(2E)-2-[(E)-({3-hydroxy-2-methyl-5-[(phosphonooxy)methyl]pyridin-4-yl}methylidene)amino]pent-2-enoic acid | C13 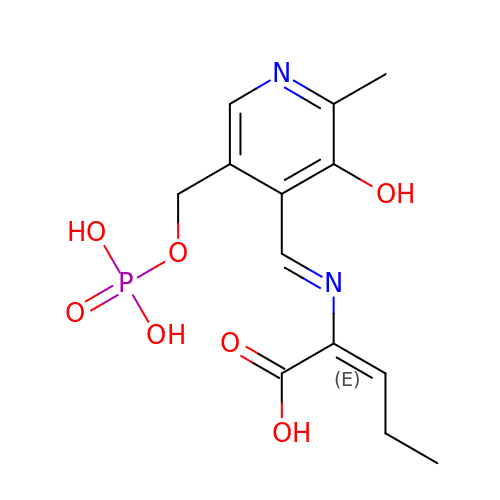H17 N2 O7 P | GKBVRDDWDGNBFQ-VVUJNEFVSA-N> APTGDPACRAAVATAQKIAPLAHGEVAALTMASAPLKLPDLAFEDADGKPKKLSDFRGKTLLVNLWATWCVPSRKEMPALDELQGKLSGPNFEV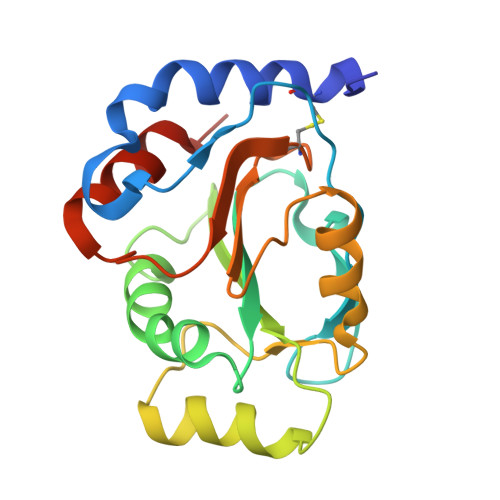VAINIDTRDPEKPKTFLKEANLTRLGYFNDQKAKVFQDLKAIGRALGMPTSVLVDPQGCEIATIAGPAEWASEDALKLIRAATGKAAAAL>QEVEFDIPPQALGSALQEFGRQADIQVLYRPEEVRNKRSSAIKGKLEPNQAITELLRGTGASVDFQGNAITISVAEAADSSVDLGATMITSNQLGTITEDSGSYTPGTIATATRLVLTPRETPQSITVVTRQNMDDFGLNNIDDVMRHTPGITVSAYDTDRNNYYARGFSINNFQYDGIPSTARNVGYSAGNTLSDMAIYDRVEVLKGATGLLTGAGSLGATINLIRKKPTHEFKGHVELGAGSWDNYRSELDVSGPLTESGNVRGRAVAAYQDKHSFMDHYERKTSVYYGILEFDLNPDTMLTVGADYQDNDPKGSGWSGSFPLFDSQGNRNDVSRSFNNGAKWSSWEQYTRTVFANLEHNFANGWVGKVQLDHKINGYHAPLGAIMGDWPAPDNSAKIVAQKYTGETKSNSLDIYLTGPFQFLGREHELVVGTSASFSHWEGKSYWNLRNYDNTTDDFINWDGDIGKPDWGTPSQYIDDKTRQLGSYMTARFNVTDDLNLFLGGRVVDYRVTGLNPTIRESGRFIPYVGAVYDLNDTYSVYASYTDIFMPQDSWYRDSSNKLLEPDEGQNYEIGIKGEYLDGRLNTSLAYFEIHEENRAEEDALYNSKPT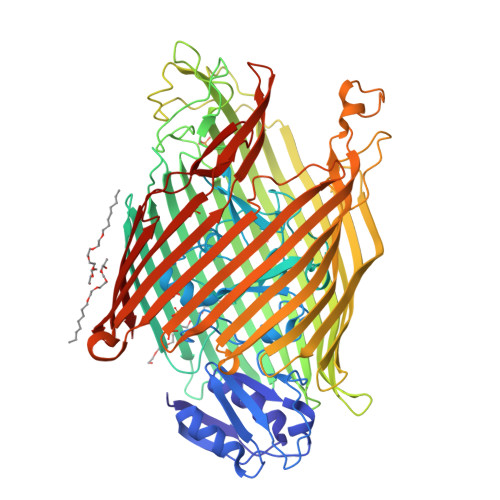NPAITYAYKGIKAKTKGYEAEISGELAPGWQVQAGYTHKIIRDDSGKKVSTWEPQDQLSLYTSYKFKGALDKLTVGGGARWQGKSWQMVYNNPRSRWEKFSQEDYWLVDLMARYQITDKLSASVNVNNVFDKTYYTNIGFYTSASYGDPRNLMFSTRWDF[2x];> SRSKKKTT2-(4-METHYLPHENOXY)ETHYLPHOSPHINATE 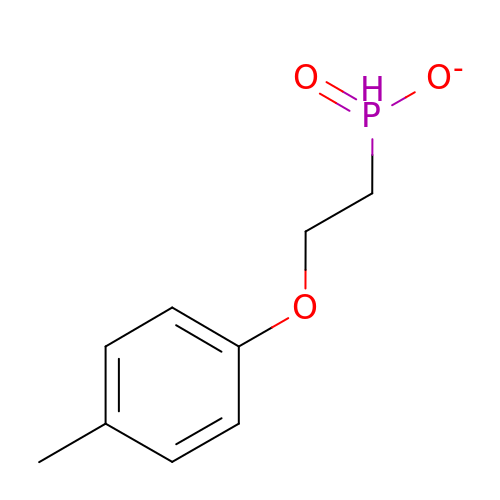| C9 H12 O3 P | SATOOOGJLDLPLZ-UHFFFAOYSA-M> MDYLKPAQKGRRRGLSINSLSETQQSAMNSSLDHLQNDLNRINLQWNRILSDNTNPLELALAFLDDTSVGLGHRYEEFNQLKSQIGSHLQDVVNEHSQVFNTNVASYGKAVSSIMQAQEQTLNLKNCLKEANEKITTDKGSLQELNDNNLKYTKMIDVLVNIEELLQIPEKIEENIRKENFHQVQILLERGFILMNNKSLKTVEILKPINQQLELQEHLLFNNLIEEIHDIMYSKSNKTNFTRVTNNDIFKIISISHNGFTSLENYLYNIVNIDIMEHSKTINKNLEQFIHDQSLNKGNIMLQENAATQAPLAPSRNQENEGFNRIGFLLKTINNINKLPVAFNIITERAKEEIHNIIVKSTESIRSKHPSLLKMATSLKNDNHFGLPVQDILSIILRECFWEIFLKLLYAIQCHRAIFEMSNILQPTSSAKPAFKFNKIWGKLLDEIELLLVRYINDPELISSNNGSIKPINGATNNAPTLPKRKNPKIFSLEYNIEDNSSVKDQAFELKALLKDIFPGFSVSSNMDLDSIYVKDESFEQDEPLVPPSVFNMKVILDPFLLFTQSTSTIVPSVLTQNTISSLTFFDDYMNKSFLPKIQMTMDYLFTVEVESNNPYALELSDENHNIFKTALDFQRLFYNLLNVFNTANTFREKISYCILDLLNHFYNYYLGLFNSLIGTSDRHLTRKIITAWLQNGILMDQEQKILNGDETLFHEESIELFKEIPHFYQAGKGLSKSDLFNNLTLDTILQFSASVLWILNWLPGLKKAINIDEVSQEPMLDADRLRSSWTFSESMDLNYSNPSSSPNSLGNLKILLDDKASKKFDETIDGFKTLKFKLITILRFNIRALCIYDIGSFFQNTKIWNMDVGSIELDQNIASLISELRRTESKLKQQLPEKEKNSIFIGLDIVNNYALIKGAKSIKVLNHNGIKKMLRNVNVLQHAYRNL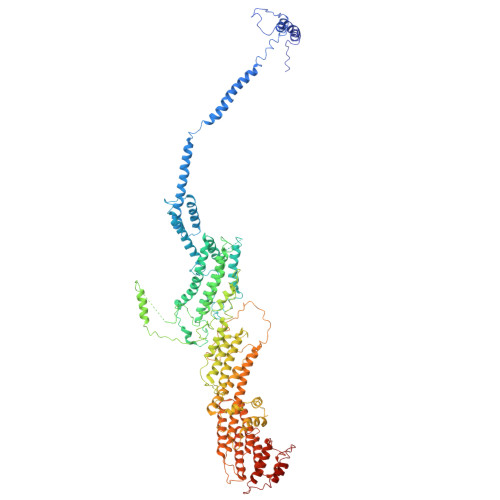SSEPSKINMNVTMNFYSLCGSSEAELFEYIKDNELPHCSVEDLKTILRLQFSEEMHRQLKRQSTSSTKGSIKPSNKRYTEALEKLSNLEKEQSKEGARTKIGKLKSKLNAVHTANEK>[2x]MAQVQPWVDEDLKDSTEDLQVEEDAEEWQEAEESVEHIPFSHTRYPEQEMRMRSQEFYELLNKRRSVRFISSEHVPMEVIENVIKAAGTAPSGAHTEPWTFVVVKDPDMKHKIREIIEEEEEINYMKRMGKRWVTDLKKLRTNWIKEYLDTAPVLILIFKQVHGFAANGKKKVHYYNEISVSIAAGLLLAA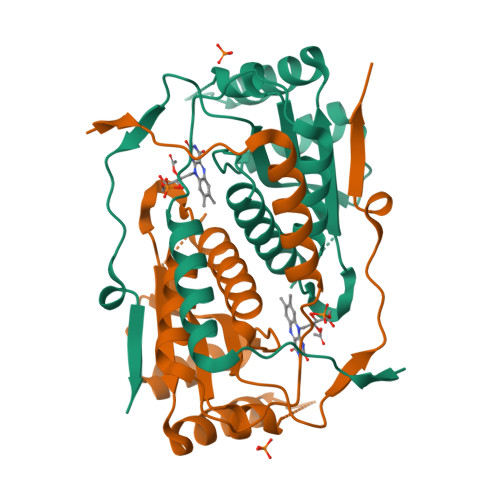LQNAGLVTVTTTPLNAGPRLRVLLGRPSHEKLLVLLPVGYPSRDATVPDLKRKALDQIMVTVHHHHHH>GSMDPLSPPLCTLPPGPEPPRFVCYCEGEESGEGDRGGFNLYVTDAAELWSTCFTPDSLAALKARFGLSAAEDITPRFRAACEQQAVALTLQEDRASLTLSGGPSALAFDLSKVPGPEAAPRLRALTLGLAK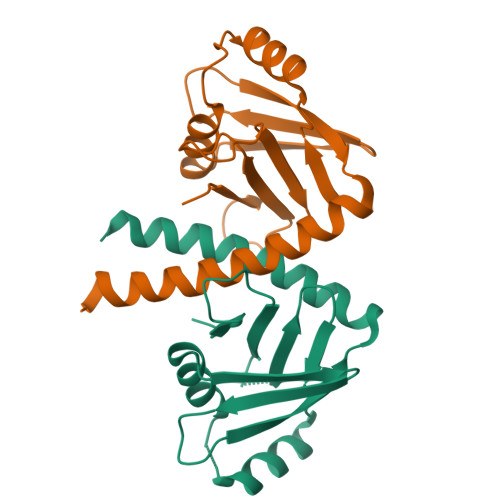RVWSLERRLAAAEETAVSPRKSPRPAGPQLFLPDPD[2x]> MNYQPIEHRGQALWLLADKAIYWPARRALLVADVHIGKAASYRALHQPVPRGTTEATLARLDRLLAEHDCEQLIILGDFLHARTARAPATLAKVEDWRKRHKNLKVVLIRGNHDRNAG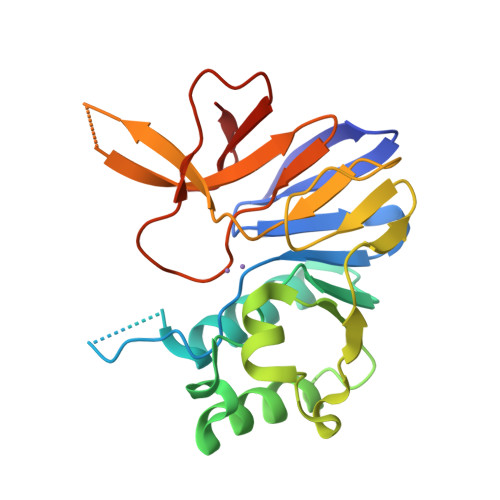DPPASLDIQVVDEPWVLEPFALQHEPQPHGTHPVLAGHVHPVFVLRGKARQRLRLPCFVIDEQVSLLPAFGEFTGGWEITPASASRLYLAGAERVWPL> GPMTDQAFVTLTTNDAYAKGALVLGSSLKQHRTTRRLVVLATPQVSDSMRKVLETVFDEVIMVDVLDSGDSAHLTLMKRPELGVTLTKLHCWSLTQYSKCVFMDADTLVLANIDDLFDREELSAAPDPGWPDCFNSGVFVYQPSVETYNQLLHLASEQGSFDGGDQGILNTFFSSWATTDIRKHLPFIYNLSSISIFSYLPAFKVFGASAKVVHFLGRVKPWNYTYDPKTKSVKSEAHDPNMTHPEFLILWWNIFTTNVLPLLQQFGLVKDTCSYVNVLSDLVYTLAFSCGFCRKEDVSGAISHLSLGEIPAMAQPFVSSEERKERWEQGQA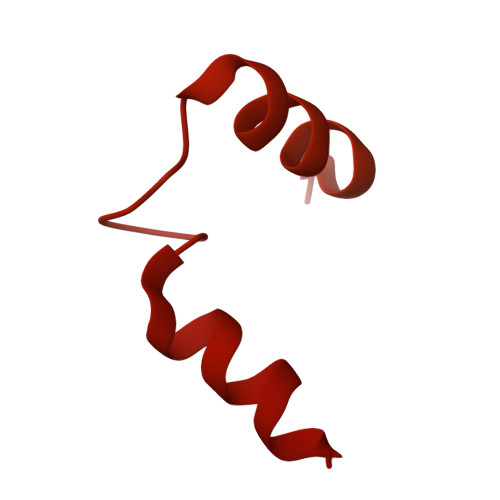DYMGADSFDNIKRKLDTYLQ7-({3-[2-(6-aminopyridin-2-yl)ethyl]phenoxy}methyl)quinolin-2-amine | C23 H22 N4 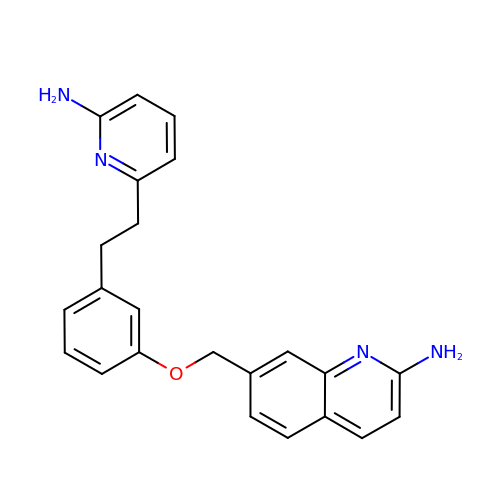O | WNELLCJMJQCVPO-UHFFFAOYSA-N> GSPALDTGTTEEDRLKIDVIDWLVFDPAQRAEALKQGNAIMRKFLASKKHEAAKEVFVKIPQDSIAEIYNQCEEQGMESPLPAEDDNAIREHLCIRAYLEAHETFNEWFKHMNSVPGGSGGSWKGHLDALTADVKEKMYNVLLFVDGGWMVDVREDAKEDHERTHQMVLLRKLC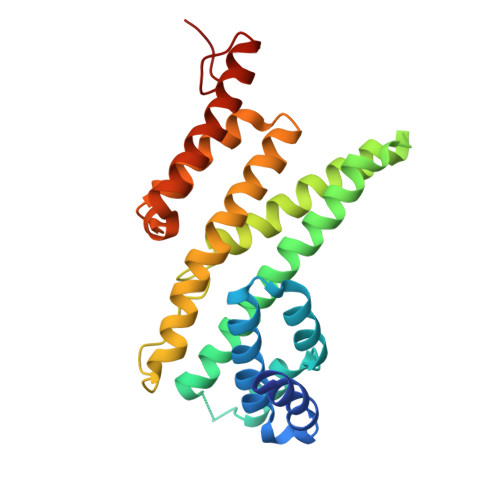LPMLCFLLHTILHSTGQYQECLQLADMVSSERHKLYLVFSKEELRKLLQKLRESSLMLLDQGLDPLGYEIQL> GAQ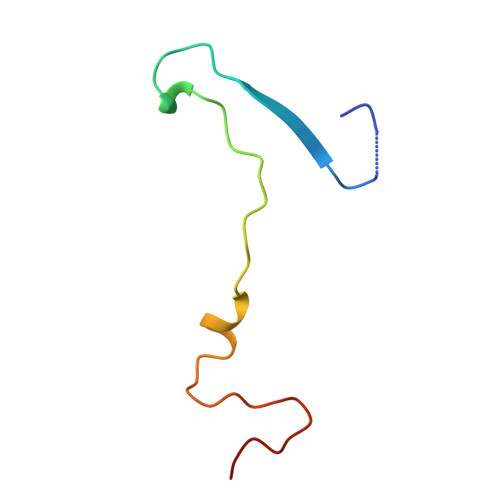GGSTINYNNINYYSHAASAAQNKQDFTQDPSKFTQPIADVIKETAVPLK> GPIQLWQFLLELLTDKSCQSFISWTGDGWEFKLSDPDEVARRWGKRKNKPKMNYEKLSRGLRYYYDKNIIHKTAGKRYVYRFVCDLQSLLG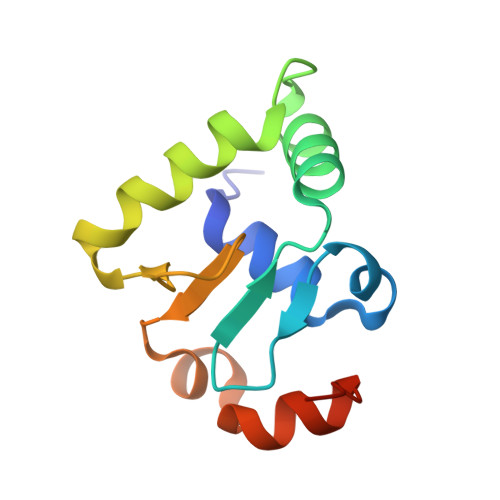YTPEELHAMLDVKPDADE>MSLKQYYMICIPKVLDDSSDFWSVLVEGAQMAAKEYEIKLEFMAPEKEEDYL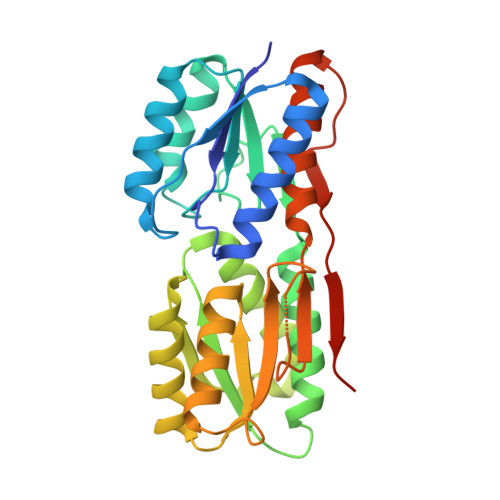VQNELIEEAIKRKPDVILLAAADYEKTYDAAKEIKDAGIKLIVIDSGMKQDIADITVATDNIQAGIRIGAVTKNLVRKSGKIGVISFVKNSKTAMDREEGLKIGLSDDSNKIEAIYYCDSNYDKAYDGTVELLTKYPDISVMVGLNQYSATGAARAIKDMSLEAKVKLVCIDSSMEQIQYLEEGIFEAMVVQKPFNIGYLGVEKALKLLKKEYVPKQLDSGCALITKDNEGHHHHHH[2x]> MDPIINGNSANVYLTDSYLKGVISFSECNALGSYIFNGPYLKNDYTNLISRQNPLIEHMNLKKLNITQSLISKYHKGEIKLEEPTYFQSLLMTYKSMTSSEQIATTNLLKKIIRRAIEISDVKVYAILNKLGLKEKDKIKSNNGQDEDNSVITTIIKDDILSAVKDNQSHLKADKNHSTKQKDTIKTTLLKKLMCSMQHPPSWLIHWFNLYTKLNNILTQYRSNEVKNHGFTLIDNQTLSGFQFILNQYGCIVYHKELKRITV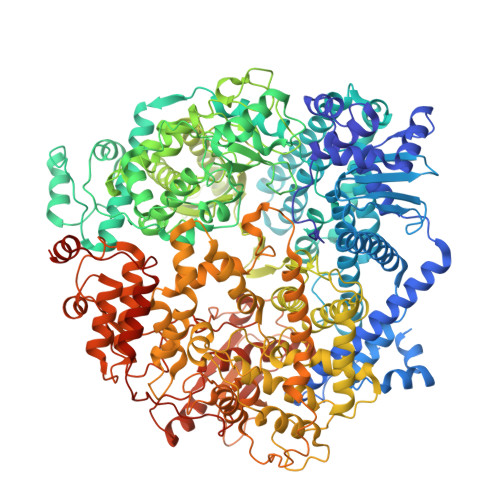TTYNQFLTWKDISLSRLNVCLITWISNCLNTLNKSLGLRCGFNNVILTQLFLYGDCILKLFHNEGFYIIKEVEGFIMSLILNITEEDQFRKRFYNSMLNNITDAANKAQKNLLSRVCHTLLDKTVSDNIINGRWIILLSKFLKLIKLAGDNNLNNLSELYFLFRIFGHPMVDERQAMDAVKINCNETKFYLLSSLSMLRGAFIYRIIKGFVNNYNRWPTLRNAIVLPLRWLTYYKLNTYPSLLELTERDLIVLSGLRFYREFRLPKKVDLEMIINDKAISPPKNLIWTSFPRNYMPSHIQNYIEHEKLKFSESDKSRRVLEYYLRDNKFNECDLYNCVVNQSYLNNPNHVVSLTGKERELSVGRMFAMQPGMFRQVQILAEKMIAENILQFFPESLTRYGDLELQKILELKAGISNKSNRYNDNYNNYISKCSIITDLSKFNQAFRYETSCICSDVLDELHGVQSLFSWLHLTIPHVTIICTYRHAPPYIGDHIVDLNNVDEQSGLYRYHMGGIEGWCQKLWTIEAISLLDLISLKGKFSITALINGDNQSIDISKPIRLMEGQTHAQADYLLALNSLKLLYKEYAGIGHKLKGTETYISRDMQFMSKTIQHNGVYYPASIKKVLRVGPWINTILDDFKVSLESIGSLTQELEYRGESLLCSLIFRNVWLYNQIALQLKNHALCNNKLYLDILKVLKHLKTFFNLDNIDTALTLYMNLPMLFGGGDPNLLYRSFYRRTPDFLTEAIVHSVFILSYYTNHDLKDKLQDLSDDRLNKFLTCIITFDKNPNAEFVTLMRDPQALGSERQAKITSEINRLAVTEVLSTAPNKIFSKSAQHYTTTEIDLNDIMQNIEPTYPHGLRVVYESLPFYKAEKIVNLISGTKSITNILEKTSAIDLTDIDRATEMMRKNITLLIRILPLDCNRDKREILSMENLSITELSKYVRERSWSLSNIVGVTSPSIMYTMDIKYTTSTISSGIIIEKYNVNSLTRGERGPTKPWVGSSTQEKKTMPVYNRQVLTKKQRDQIDLLAKLDWVYASIDNKDEFMEELSIGTLGLTYEKAKKLFPQYLSVNYLHRLTVSSRPCEFPASIPAYRTTNYHFDTSPINRILTEKYGDEDIDIVFQNCISFGLSLMSVVEQFTNVCPNRIILIPKLNEIHLMKPPIFTGDVDIHKLKQVIQKQHMFLPDKISLTQYVELFLSNKTLKSGSHVNSNLILAHKISDYFHNTYILSTNLAGHW>GSSHHHHHHSSGLVPRGSHMASAQETTRLTATEIRARISEGAASREEVVHEHLDRIDEFNALTNSFVELRADQVLEEARAADREFGSTLGGPLDGVPLSIKDSYSVAGLHRTDGLPVNADVLDAQDDVATARLRAAGGLVLGHAGIPDLCIRWNSVSGLYGAVRNPRDLSRTAGGSSGGDAANVAAGFATIGLGGDLGGSIRVPASWCGVYGFRTGPGRIPDVNPNGGRSRNVVMELMAQIGPIARSIDDIELAFRIMTGVDRRDTMSSPLGLIEPIEAPRVAVLRHETGAVLDSSVEEQLDATIEMLRAEGYVVEENVLPDLHRAPEVWAEIVGTELIHRVL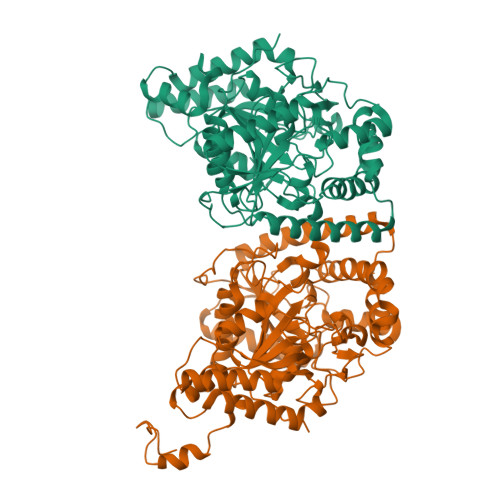PEVAELVIASERMHIVDMFGAYELGADVGAYLTALEERSSIQMTVAALMERYQLILAPVAGMPAPPLDFDDHIGREASIALFDQMRCVPWVNLLGLPSLALPNGIQLVGRKHDELTILAAGRAYERRAPRVEIATPAI[2x]> MASHHHHHHSGMEEWNFPVEYDENYLPPADSRYWFPRRETMPAAERDKAILGRLQQVCQYAWEHAPFYRRKWEEAGFQPSQLKSLEDFEARVPVVKKTDLRESQAAHPPFGDYVCVPNSEIFHVHGTSGTTGRPTAFGIGRADWRAIANAHARIMWGMGIRPGDLVCVAAVFSLYMGSWGALAGAERLRAKAFPFGAGAPGMSARLVQWLDTMKPAAFYGTPSYAIHLAEVAREEKLNPRNFGLKCLFFSGEPGASVPGVKDRIEEAYGAKVYDCGSMAEMSPFMNVAGTEQSNDGMLCWQDIIYTEVCDPANMRRVPYGQRGTPVYTHLERTSQPMIRLLSGDLTLWTNDENPCGRTYPRLPQGIFGRIDDMFTIRGENIYPSEIDAALNQMSGYGGEHRIVITRESAMDELLLRVEPSESVHAAGAAALETFRTEASHRVQTVLGVRAKVELVAPNSIARTDFKARRVIDDREVFRALNQQLQSSAGSAWSHPQ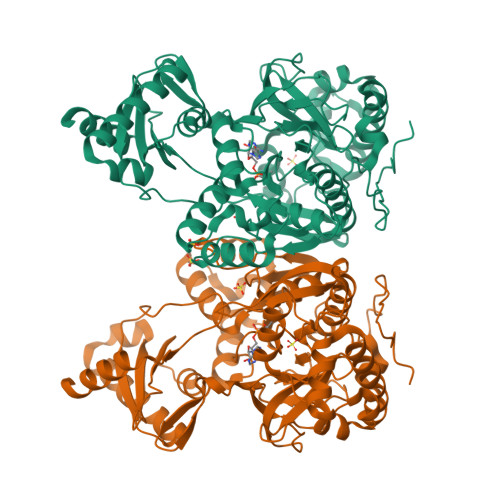FEK> HMAASCVLLHTGQKMPLIGLGTWKSEPGQVKAAIKYALTVGYRHIDCAAIFGNELEIGEALQETVGPGKAVPREELFVTSKLWNTKHHPEDVEPALRKTLADLQLEYLDLYLMHWPYAFERGDNPFPKNADGTIR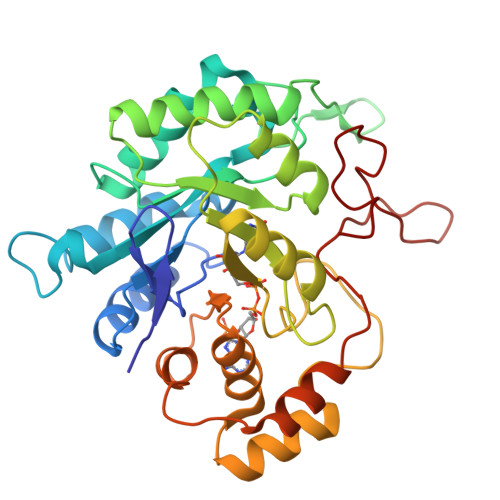YDATHYKDTWKALEALVAKGLVRALGLSNFSSRQIDDVLSVASVRPAVLQVECHPYLAQNELIAHCQARGLEVTAYSPLGSSDRAWRDPNEPVLLEEPVVQALAEKYNRSPAQILLRWQVQRKVICIPKSVTPSRIPQNIQVFDFTFSPEEMKQLDALNKNLRFIVPMLTVDGKRVPRDAGHPLYPFNDPY> KKK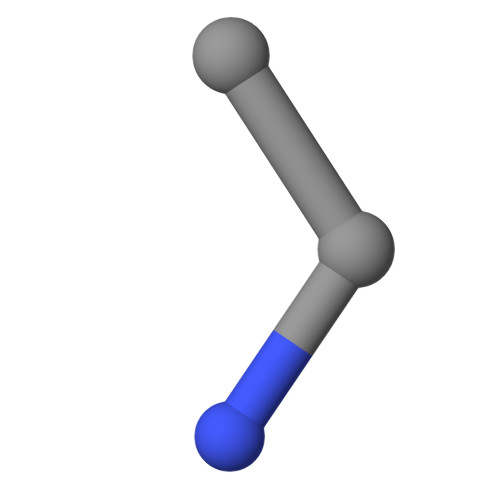K>TDTTPPTITVPSDIIAYRGEEFEFYFEITDDSGQ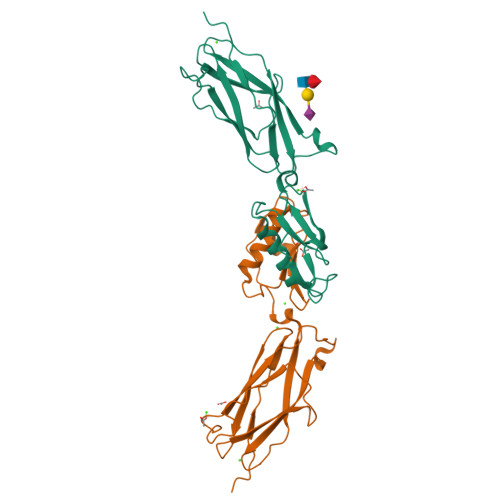VKNIELSTFGKPLGLNWLEYSEDNFNVPGNATSDNPLRVRVHGTVPLNEPIPADKNRAQFTRTIRAWDAAGNVSSNITFVIKYRAQTDKYNPADPTITYVDRLSSLSPSEKNAVEAAVRAANPQIPAAARITVSANGTVTITYPDSSTDTITANRVVKDLASS[2x]> MMDRTRLFLAAEFKQKSRWSSVWPNMHYGAMYLSYSIGRKLPMKGVNWVTRESNRLTNFSNRYQAVINDIDVKKTEEELGITLQDIRWNDHRRIYWKCSFCGSSYRKSVSVRTKFHAGCNFCKGRYPSEVLREQHQSLSLAASAPELIKQLKETDKKDNLGSLALTSKFRAEWKCQSCGGSYRASVRSRTGMVENGQCPLHPNIVDWSAYCPSCSWRPNMEAIAEEVQRTGQFLGLEAESRKIASAPPARIPRRKK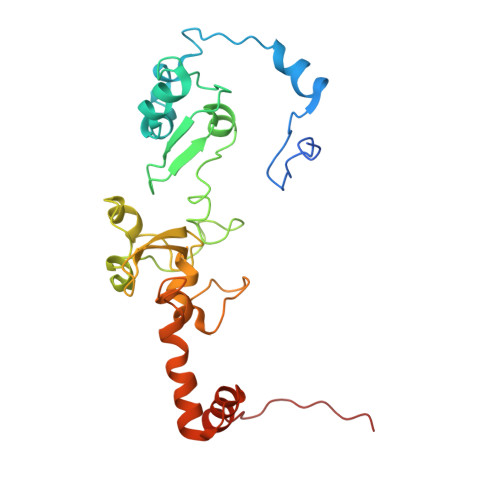LVS Carbamoyltransferases (CTases) catalyze carbamoylation, an important modification for the bioactivity of many secondary metabolites with pharmaceutical applications. GdmN and Asm21 contribute to O-carbamoylation at the C7 (S configuration) of geldanamycin and ansamitocins, respectively. CTases in class III, which modify secondary metabolites, adopt two nucleophilic half-reactions, the formation of carbamoyl-AMP derived from ATP, CP, and Mg2+ and the subsequent transfer of the carbamoyl group from carbamoyl-AMP to the secondary metabolites. GdmN forms a face-to-face homodimer through unusual C-terminal domains, a previously unknown functional form for CTases.

Therefore, the co-crystal structures of GdmN/AMP/1 (2.80 Å resolution), GdmN/ATP (2.00 Å resolution), and GdmN/carbamoyl-AMP (1.98 Å resolution) were determined. The electron density clearly revealed that 1, CP, carbamoyl-AMP, and the nucleotides were bound in different substrate-binding sites. In the GdmN/AMP/1, GdmN/ATP, and GdmN/carbamoyl-AMP complexes, the electron density of AMP, ATP, or carbamoyl-AMP only appears in the subdomain of the Kae1-like domain, and these compounds make similar contacts with surrounding residues to those with TobZ. Further experiments indicated that GdmN shares a similar adenylation mechanism with TobZ. Carbamoyl-AMP appears to surround the iron ion binding site, with the amine of the carbamoyl group coordinated to iron ion and the carbonyl oxygen accommodated by the conventional oxyanion hole composed of the backbone amides of R158 and G15732. Subsequently, the docking studies using the GdmN/carbamoyl-AMP complex and 3 suggested that GdmN would be unable to bind 3 in the expected orientation, as we assumed that 3 might have steric interference with loop 2 (D156-H162).

>MLVLGLNGNFSAADTDVVPQLGEVFFHDSAASLIRDGELVAAVEEERLNRIKKTTKFPLNAVRECLALAGARPEDVDAVGYYFPENHIDTVLNHLYTEYPRAPLRYSRELIRQRLKEGLGWDLPDEKLVYVPHHEAHAYSSYLHSGMDSALVLVLDGRGELHSGTVYRAEGTRLEKLADYPVPKSLGGLYLNATYLLGYGFGDEYKVMGLAPWGNPETYRDTFAKLYTLQDNGEYELHGNIMVPNLVSPLFYAEGFRPRRKGEPFTQAHRDFAAALQETVEKIVLHILEYWAKTSGHSRLCFGGGVAHNSSLNGLILKSGLFDEVFVHPASHDAGAGEGAAYAAAASLGTLERPGKRLLSASLGPALGGREQIRARLADWAPLIDVEFPDDAVETAAGLLAEGQVLGWAYGRSEFGPRALGHRSIVADARPEENRTRINAMVKKREGFRPFAPVVTAEAARDYFDLSGADGNHEFMSFVVPVLPERRTELGAVTHVDGTARVQVVSAESGERFHRLVRRFGELTGTPVLLNTSFNNNAEPIVQSLDDVVTSFLTTDLDVLVVEDCLVRGKASPDLGVLVPRFRPVTRLVERRTAGPDASAGAKTHEIHLDYDGGPSAKVSPELYELLGAVDGTTTLGDLAKTVGGLSDALATEVFALWEQRFLTLAPAGDIGPLADDGTRGH[2x]> MSMILKEIRMNNFKSHVNSRIKFEKGIVAIIGENGSGKSSIFEAVFFALF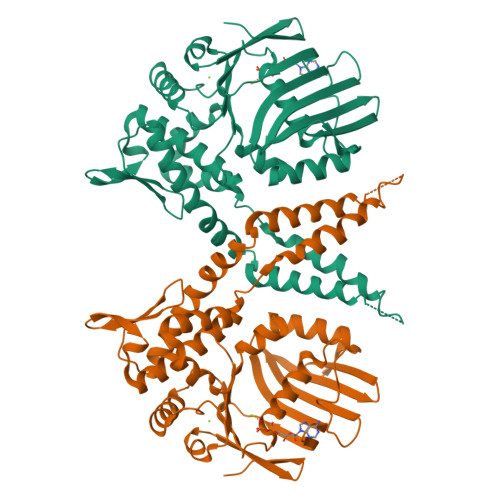GAGSNFNYDTIITKGKKSVYVELDFEVNGNNYKIIREYDSGRGGAKLYKNGKPYATTISAVNKAVNEILGVDRNMFLNSIYIKQGEIAKFLSLKPSEKLETVAKLLGIDEFEKCYQKMGEIVKEYEKRLERIEGELNYKEESLKARLKEMSNLEKEKEKLTKFVEYLDKVRRIFGRNGFQAYLREKYVPLIQKYLNEAFSEFDLPYSFVELTKDFEVRVHAPNGVLTIDNLSGGEQIAVALSLRLAIANALIGNRVECIILDEPTVYLDENRRAKLAEIFRKVKSIPQMIIITHHRELEDVADVIINVKKDGNVSKVKING> MADHKKVVDHYENPRNVGSLDKTSKNVGTGLVGAPACGDVMKLQIQVDEKGKIVDARFKTFGCGSAIASSSLATEWVKGKTVEEALTIKNTDIAKELCLPPVKLHCSMLAEDAIKAALADYKLKQEPKKGEAEKK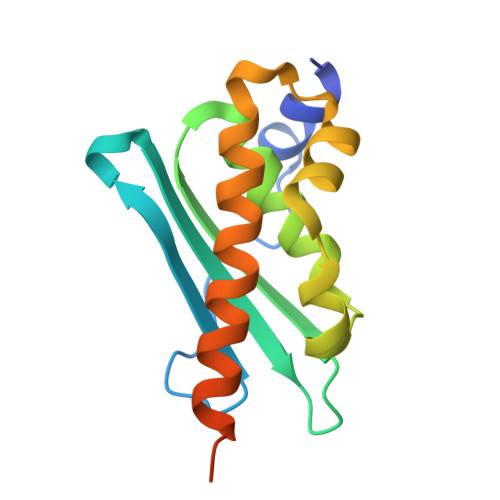LEHHHHHH>GTITAVKGGVKKQLKFEDDQTLFTVLTEAGLMSADDTCQGNKACGKCICKHVSGKVAAAEDDEKEFLEDQPANARLACAITLSGENDGAVFEL[3x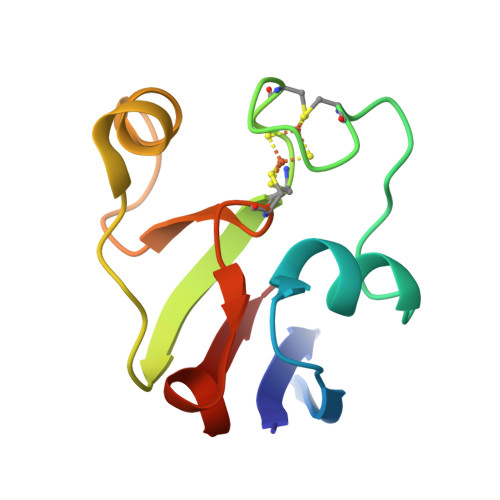]(2S)-2-[({3-hydroxy-2-methyl-5-[(phosphonooxy)methyl]pyridin-4-yl}methyl)amino]but-3-enoic 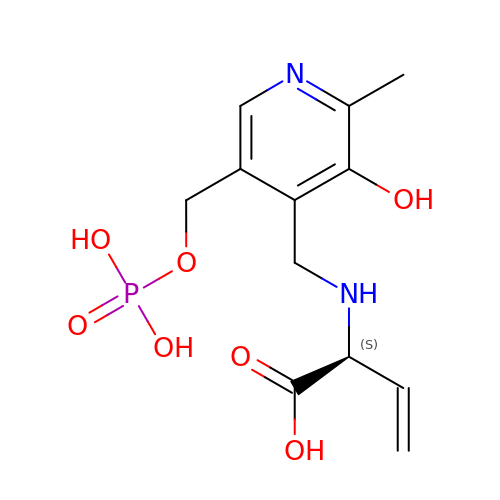acid | C12 H17 N2 O7 P | HVUNMKYNYWDWQK-JTQLQIEISA-N11-[(2R,3S)-3-PENTYLOXIRAN-2-YL]UNDECANOIC 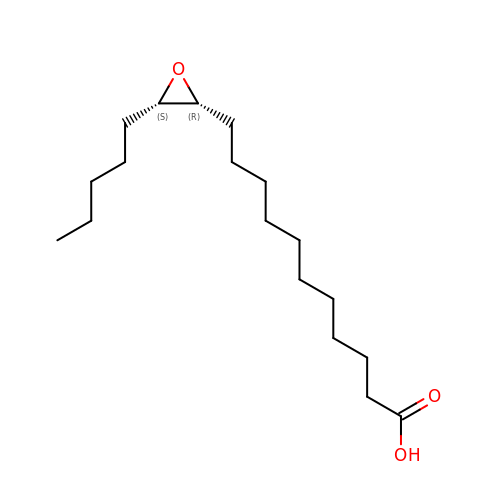ACID | C18 H34 O3 | AHXFZOAYPPCFEB-DLBZAZTESA-N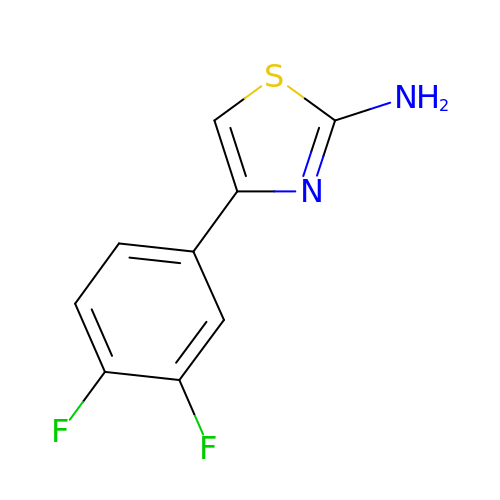4-[3,4-bis(fluoranyl)phenyl]-1,3-thiazol-2-amine | C9 H6 F2 N2 S | NDCSJUJQMRFHEX-UHFFFAOYSA-N2-[(3R)-3-aminopiperidin-1-yl]-3-(but-2-yn-1-yl)-5-[(4-methylquinazolin-2-yl)methyl]-3H-imidazo[2,1-b]purin-4(5H)-one 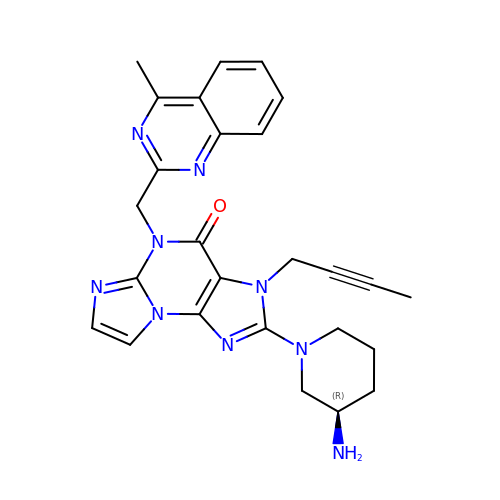| C26 H27 N9 O | MQXMHDINDWMFHK-GOSISDBHSA-N>GSNKLHLRVVTLIEHPFVFTREVDDEGLCPAGQLCLDPMTNDSSMLDRLFSSLHSSNDTVPIKFKKCCYGYCIDLLEQLAEDMNFDFDLYIVGDGKYGAWKNGHWTGLVGDLLSGTANMAVTSFSINTARSQVIDFTSPFFSTSLGILVRTRGTELSGIHDPKLHHPSQGFRFGTVRESSAEDYVRQSFPEMHEYMRRYNVPATPDGVQYLKNDPEKLDAFIMDKALLDYEVSIDADCKLLTVGKPFAIEGYGIGLPPNSPLTSNISELISQYKSHGFMDVLHD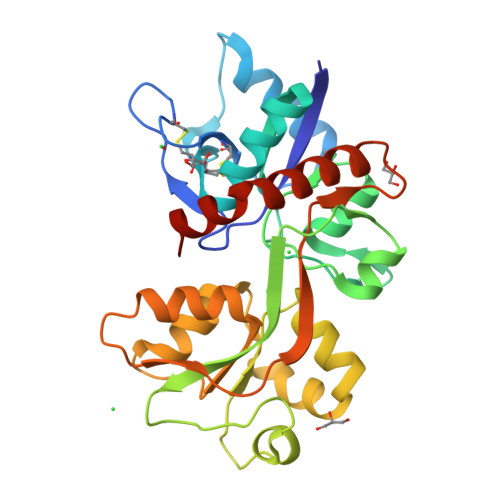KWYKVVPCGK[2x]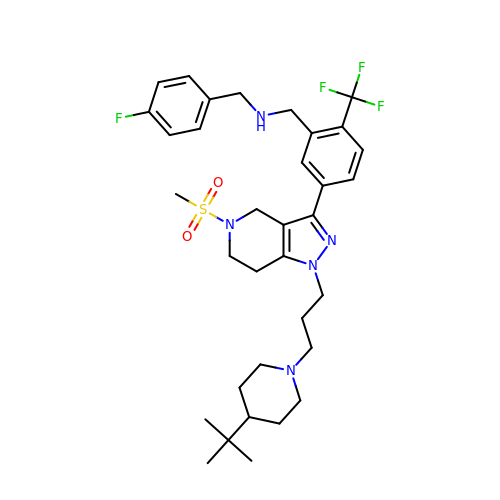1-[5-{1-[3-(4-tert-butylpiperidin-1-yl)propyl]-5-(methylsulfonyl)-4,5,6,7-tetrahydro-1H-pyrazolo[4,3-c]pyridin-3-yl}-2-(trifluoromethyl)phenyl]-N-[(4-fluorophenyl)methyl]methanamine | C34 H45 F4 N5 O2 S | CJOOHSAYHGMMHB-UHFFFAOYSA-N> GEESRNTTVLDTTTTLQSSGFGRAFFGEAFNDLKTLMRRYQLYGQLLLSVTTDKDIDHCMFTFPCLPQGLALDIGSAGSPHEIFNRCRDGIIPLIASGYRFYRGDLRYKIVFPSNVNSNIWVQHRPDRRLEGWSAAKIVNCDAVSTGQGVYNHGYASHIQITRVNNVIELEVPFYNATCYNYLQAFNASSAASSYAVSLGEISVGFQATSDDIASIVNKPVTIYYSIGDGMQFSQWVGYQPMMILDQLPAPVVRAVPE;> MDNPNPGPDGEGEVELEKDSNVVLTTQRDPSTSIPAPVSVKWSRWTSNDVVDDYATITSRWYQIAEFVWSKDDP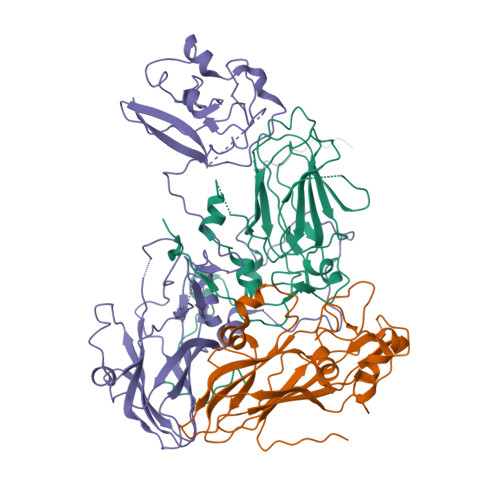FDKELARLILPRALLSSIEANSDAICDVPNTIPFKVHAYWRGDMEVRVQINSNKFQVGQLQATWYYSDHENLNISSKRSVYGFSQMDHALISASASNEAKLVIPFKHVYPFLPTRIVPDWTTGILDMGALNIRVIAPLRMSATGPTTCNVVVFIKLNNSEFTGTSSGKFYASQIRAKPE;> DNPSYQQSPRHFVPTGMHSLALGTNLVEPLHALRLDAAGTTQHPVGCAPDEDMTVSSIASRYGLIRRVQWKKDHAKGSLLLQLDADPFVEQRIEGTNPISLYWFAPVGVVSSMFMQWRGSLEYRFDIIASQFHTGRLIVGYVPGLTASLQLQMDYMKLKSSSYVVFDLQESNSFTFEVPYVSYRPWWVRKYGGNYLPSSTDAPSTLFMYVQVPLIPMEAVSDTIDINVYVRGGSSFEVCVPVQPSLGLNWNTDFILRNDEEYRAKTGYAPYYAGVWHSFNNSNSLVFRWGSASDQIAQWPTISVPRGELAFLRIKDGKQAAVGTQPWRTMVVWPSGHGYNIGIPTYNAERARQLAQHLYGGGSLTDEKAKQLFVPANQQGPGKVSNGNPVWEVMRAPLATQRAHIQDFEFIEAIPE> GPMDTKFKDDLFRKYVQFHESKVDTTTSRQRPGSDECLRVAASTLLSLHKVDPFYRFRLIQFYEVVESSLRSLSS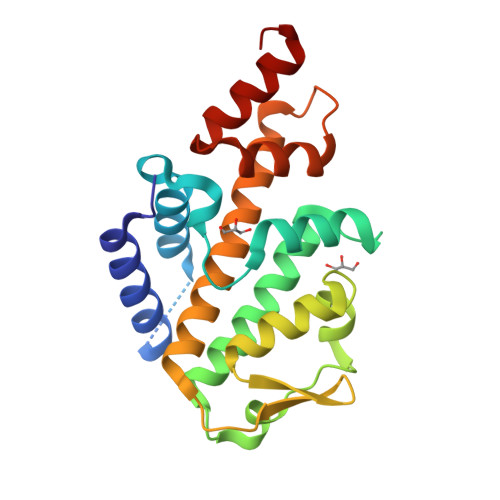SSLRALHGAFSMLETVGINLFLYPWKKEFRSIKTYTGPFVYYVKSTLLEEDIRAILSCMGYTPELGTAYKLRELVETLQVKMVSFELFLAKVECEQMLEIHSQVKDKGYSELDIVSERKSSAEDVRGCSDALRRRAEGRE>[2x]MPGLFLTLEGLDGSGKTTQARRLAAFLEAQGRPVLLTREPGGGLPEVRS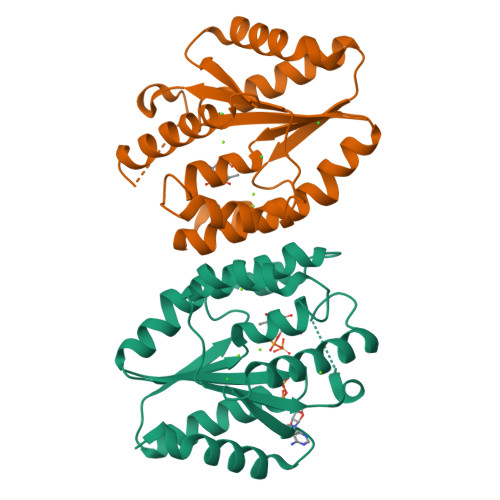LLLTQELSPEAEYLLFSADRAEHVRKVILPGLAAGKVVISDRYLDSSLAYQGYGRGLPLPWLREVAREATRGLKPRLTFLLDLPPEAALRRVRRPDRLEGLGLEFFRRVREGYLALARAEPGRFVVLDATLPEEEIARAIQAHLRPLLP> GSHVANSVLFPCKYASSGCEITLPHTEKADHEELCEFRPYSCPCPGASCKWQGSLDAVMPHLMHQHKSITTLQGEDIVFLATDINLPGAVDWVMMQSCFGFHFMLVLEKQEKYDGHQQFFAIVQLIGTRKQAENFAYRL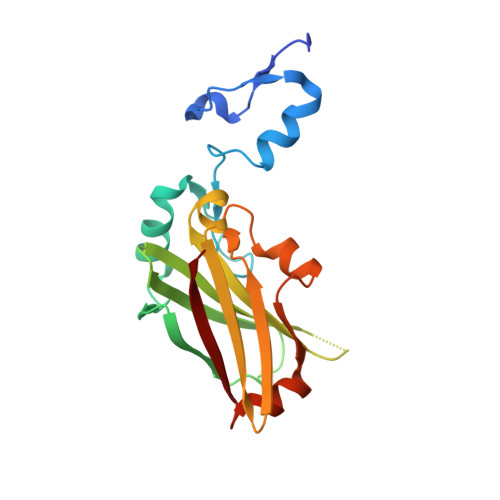ELNGHRRRLTWEATPRSIHEGIATAIMNSDCLVFDTSIAQLFAENGNLGINVTISMC The viral trans-activator of transcription (Tat) protein uses an archetypal arginine-rich motif (ARM) to recruit the host positive transcription elongation factor b (pTEFb) complex onto the viral trans-activation response (TAR) RNA, leading to activation of HIV transcription. Using yeast display and multiple rounds of selection, a new class of TAR-binding proteins (TBPs) was identified that bind TAR with nanomolar affinity. Here, we present four co-crystal structures of lab-evolved TAR-binding proteins (TBPs) in complex with HIV-1 TAR. Although it was hypothesized originally that each TBP variant would recognize TAR using fundamentally different modes of binding, we demonstrated here that each TBP binds TAR using a conserved subset of arginine-to-guanine interactions within a lab-evolved β2-β3 loop.

ITC revealed high-affinity TAR binding based on a KD of 4.2 ± 0.3 nm. Despite only three arginines, we hypothesized that this variant would possess strong affinity comparable with TBP6.7 or TBP6.9 because each threonine has the ability to form hydrogen bonds that stabilize the β2-β3 loop backbone. As expected, the co-crystal structure revealed an interaction between Oγ1 of Thr-48 and the carbonyl oxygen of Thr-50 (Fig. 3 (F and I) and Fig. S3A), as observed for TBP6.7 and TBP6.9. A second interaction is also shared among TBP6.7, TBP6.9, and TBP6.6. Each protein makes a hydrogen bond between Oγ1 of Thr-50 and Nε of Arg-52, stabilizing a favorable arginine rotamer for guanine recognition (Figs. 2B and 3 (E and F) and Fig. S3B). A main take-home message for TBP6.6 is that stabilization of the β2-β3 loop by threonine-mediated intramolecular hydrogen bonding is favorable. TBP6.6's ΔΔG° of −0.2 kcal mol−1 is slightly more favorable compared with TBP6.7, and its ΔG° is equivalent to TBP6.9. These observations provide a rationale for the preference of threonine at positions 48 and 50 and how glutamine and arginine are tolerated at position 48, whereas arginine is not well-tolerated at position 50.

> AVPETRPNHTIYINNLNSKIKKDELKKSLHAIFSRFGQILDILVPRTRTPRGQAFVIFKEVSSATNALRSMQGFPFYDKPMAIQYAKTDKRIP>MSFVDHPPDWLEEVGEGLREFLGLEAGPPKPKPNQQHQDQARGLVLPGYNYLGPGNGLDRGEPVNRADEVAREHDISYNEQLEAGDNPYLKYNHADAEFQEKLADDTSFGGNLGKAVFQAKKRVLEPFGLVEEGAKTAPTGKRIDDHFPKRKKARTEEDSKPSTSSDAEAGPSGSQQLQIPAQPASSLGADTMSAGGGGPLGDNNQGADGVGNASGDWHCDSTWMGDRVVTKSTRTWVLPSYNNHQYREIKSGSVDGSNANAYFGYSTPWGYFDFNRFHSHWSPRDWQRLINNYWGFRPRSLRVKIFNIQVKEVTVQDSTTTIANNLTSTVQVFTDDDYQLPYVVGNGTEGCLPAFPPQVFTLPQYGYATLNRDNTENPTERSSFFCLEYFPSKMLRTGNNFEFTYNFEEVPFHSSFAPSQNLFKLANPLVDQYLYRFVSTNNTGGVQFNKNLAGRYANTYKNWFPGPMGRTQGWNLGSGVNRASVSAFATTNRMELEGASYQVPPQPNGMTNNLQGSNTYALENTMIFNSQPANPGTTATYLEGNMLITSESETQPVNRVAYNVGGQMATNNQSSTTAPATGTYNLQEIVPGSVWMERDVYLQGPIWAKIPETGAHFHPSPAMGGFGLKHPPPMMLIKNTPVPGNITSFSDVPVSSFITQYSTGQVTVEMEWELKKENSKRWNPEIQYTNNYNDPQFVDFAPDSTGEYRTTRPIGTRYLTRPL[60x]

Adeno-associated virus (AAV) are small, non-pathogenic, single-stranded DNA viruses classified in the Parvoviridae family, the Parvovirinae subfamily, and the Dependoparvovirus genus. The AAVs package a ~4.7 kilobase (kb) genome in a non-enveloped, icosahedral (T = 1) capsid with a diameter of ~260 Å. The assembled capsid is comprised of 60 monomers in an approximate ratio of 1:1:10 of VP1:VP2:VP3 (7, 8). VP3 is responsible for assembling the body of the capsid, which functions to transport and protect the viral genome.

To generate these populations, purified AAV5 capsids were incubated for 30 min at 4°C, 55°C, and 80°C prior to vitrification. At 4°C, most capsids, ~96%, contain packaged genome. The gross capsid morphology is conserved across the three temperatures. At 4°C and 55°C, density was observed between adjacent DE loops. At the center of the threefold, a basket-like density is observed at 4°C, 55°C, and 80°C. The DNA binding pocket is situated below and adjacent to this density and is comprised of amino acids E417, V419, P420, D609, H630, P631, and S632 which have been shown to interact with a nucleotide between P420 and P631 (26). DNA is modeled in the AAV5 structures at 4°C and 55°C, but the density is not observed at 80°C. Residues H619, P620, S621, and P622 are adjacent to the modeled nucleotide at 4°C and 55°C, providing similar side chains as the DNA binding region. At 4°C, a nucleotide has been modeled at the twofold interface situated in between the unresolved density and residues T223, W224, M225, G226, R289, and L290.ADENYLATE-3'-PHOSPHATE-[[2'-DEOXY-URIDINE-5'-PHOSPHATE]-3'-PHOSPHATE] 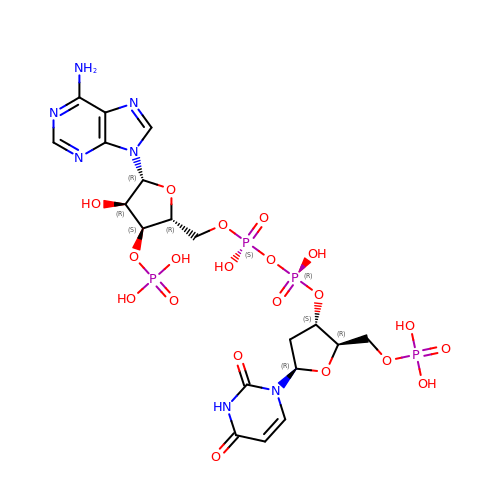| C19 H27 N7 O20 P4 | JIAJERGOUFOENU-LNAOLWRRSA-N>[2x]ASAWPEEKNYHQPAILNSSALRQIAEG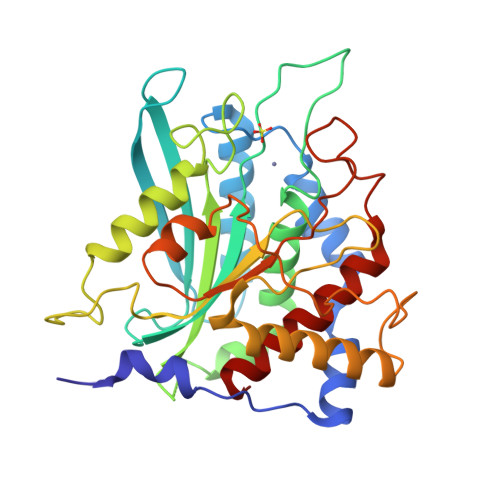TSISEMWQNDLQPLLIERYPGSPGSYAARQHIMQRIQRLQADWVLEIDTFLSQTPYGYRSFSNIISTLNPTAKRHLVLACHYDSKYFSHWNNRVFVGATDSAVPCAMMLELARALDKKLLSLKTVSDSKPDLSLQLIFFDGDEAFLHWSPQDSLYGSRHLAAKMASTPHPPGARGTSQLHGMDLLVLLDLIGAPNPTFPNFFPNSARWFERLQAIEHELHELGLLKDHSLEGRYFQNYSYGGVIQDDHIPFLRRGVPVLHLIPSPFPEVWHTMDDNEENLDESTIDNLNKILQVFVLEYLHL> MKRPVTGKDLMIVNMGPHHPSMHGVLRLIVTLDGEDVVDCEPILGYLHRGMEKIAENRAIIQYLPYVTRWDYLATMFTEAITVNGPEQLGNIQVPKRASYIRVIMLELSRIASHLLWLGPFMADIGAQTPFFYIFREREFVYDLFEAATGMRMMHNFFRIGGIAADLPYGWIDKCLDFCDYFLTEVVEYQKLITRNPIFLERVEGVGIIGGEEAINWGLSGPMLRASGIPWDLRKIDRYESYDEFEWEIQWQKQGDSLARYLVRLSEMTESIKIIQQALEGLPGGPYENLESRGFDRKRNPEWNDFEYRFISKKPSPTFELSKQELYVRVEAPKGELGIFLIGDQSGFPW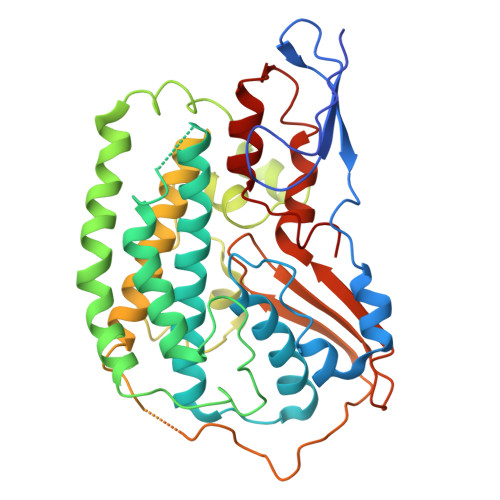RWKIRPPGFINLQILPELVKRMKLADIMTILGSIDIIMGEVDR>GSMSSERVLSYAPAFKSFLDTSFFQELSRLKLDVLKLDSTCQPLTVNLDLHNIPKSADQVPLFLTNRSFEKHNNKRTNEVPLQGSIFNFNVLDEFKNLDKQLFLHQRALECWEDGIKDINKCVSFVIISFADLKKYRFYYWLGVPCFQRPSSTVLHVRPEPSLKGLFSKCQKWFDVNYSKWVCILDADDEIVNYDKCIIRKTKVLAIRDTSTMENVPSALTKNFLSVLQYDVPDLIDFKLLIIRQNEGSFALNATFASIDPQSSSSNPDMKVSGWERNVQGKLAPRVVDLSSLLDPLKIADQSVDLNLKLMKWRILPDLNLDIIKNTKVLLLGAGTLGCYVSRALIAWGVRKITFVDNGTVSYSNPVRQALYNFEDCGKPKAELAAASLKRIFPLMDATGVKLSIPMIGHKLVNEEAQHKDFDRLRALIKEHDIIFLLVDSRESRWLPSLLSNIENKTVINAALGFDSYLVMRHGNRDEQSSKQLGCYFCHDVVAPTDSLTDRTLDQMCTVTRPGVAMMASSLAVELMTSLLQTKYSGSETTVLGDIPHQIRGFLHNFSILKLETPAYEHCPACSPKVIEAFTDLGWEFVKKALEHPLYLEEISGLSVIKQEVER[2x];>[2x]GSMIRSTLSSWREYLTPITHKSTFLTTGQITPEEFVQAGDYLAHMFPTWKWNEESSDISYRDFLPKNKQFLIIRKVPADKRAEQAVEVEGPDVIMKGFAEDGDEDDVLEYIGSETEHVQSTPAGGTKDSSIDDIDELIQDMEIKEE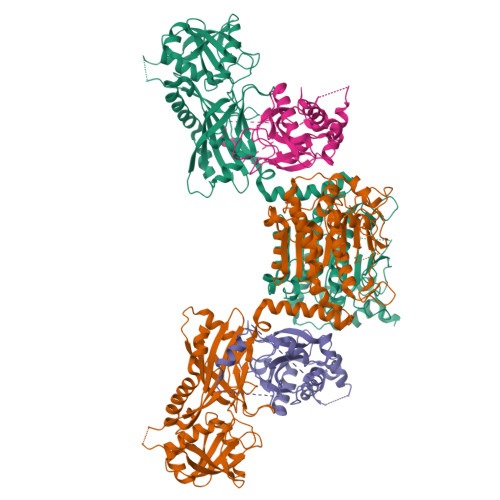DENDDTEEFNAKGGLAKDMAQERYYDLYIAYSTSYRVPKMYIVGFNSNGSPLSPEQMFEDISADYRTKTATIEKLPFYKNSVLSVSIHPCKHANVMKILLDKVRVVRQRRRKELQEEQELDGVGDWEDLQDDIDDSLRVDQYLIVFLKFITSVTPSIQHDYTMEGW>[2x]MRGSHHHHHHGSSTRSTGVENSGAGPTSFKTMKVIDPQ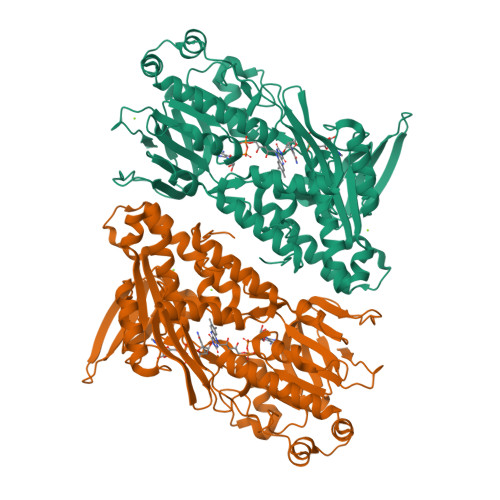HSDKPNVLILGSGWGAISFLKHIDTKKYNVSIISPRSYFLFTPLLPSAPVGTVDEKSIIEPIVNFALKKKGNVTYYEAEATSINPDRNTVTIKSLSAVSQLYQPENHLGLHQAEPAEIKYDYLISAVGAEPNTFGIPGVTDYGHFLKEIPNSLEIRRTFAANLEKANLLPKGDPERRRLLSIVVVGGGPTGVEAAGELQDYVHQDLRKFLPALAEEVQIHLVEALPIVLNMFEKKLSSYAQSHLENTSIKVHLRTAVAKVEEKQLLAKTKHEDGKITEETIPYGTLIWATGNKARPVITDLFKKIPEQNSSKRGLAVNDFLQVKGSNNIFAIGDNAFAGLPPTAQVAHQEAEYLAKNFDKMAQIPNFQKNLSSRKDKIDLLFEENNFKPFKYNDLGALAYLGSERAIATIRSGKRTFYTGGGLMTFYLWRILYLSMILSARSRLKVFFDWIKLAFFKRDFFKGL> AQTPAFDKPKVELHVHLDGAIKPETILYYGKRRGIALPADTPEELLNIIGMDKPLTLPDFLAKFDYYMPAIAGCRDAIKRIAYEFVEMKAKDGVVYVEVRYSPHLLANSKVEPI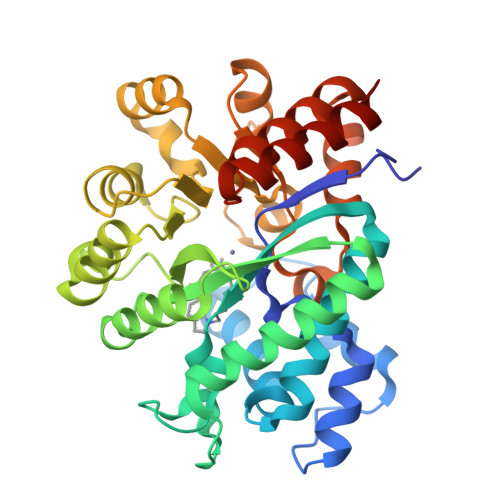PWNQAEGDLTPDEVVSLVNQGLQEGERDFGVKVRSILCCMRHQPSWSSEVVELCKKYREQTVVAIDLAGDETIEGSSLFPGHVQAYAEAVKSGVHRTVHAGEVGSANVVKEAVDTLKTERLGHGYHTLEDTTLYNRLRQENMHFEICPWSSYLTGAWKPDTEHAVIRFKNDQVNYSLNTDDPLIFKSTLDTDYQMTKKDMGFTEEEFKRLNINAAKSSFLPEDEKKELLDLLYKAYRMPSPA> GSPAKIKIVAPLESALIPGGETYQLRCDIMSTPAATIHWKFNGKLIQGSNELNVEEKLLNFGKAIVDTGIVASILTIQCPSAENSGTYSCVGYNGHQTIETVAEVEIEGEASGCRSNHKSAPEIVFWTDSRFEMTGNVATLVCRANQQVDWVW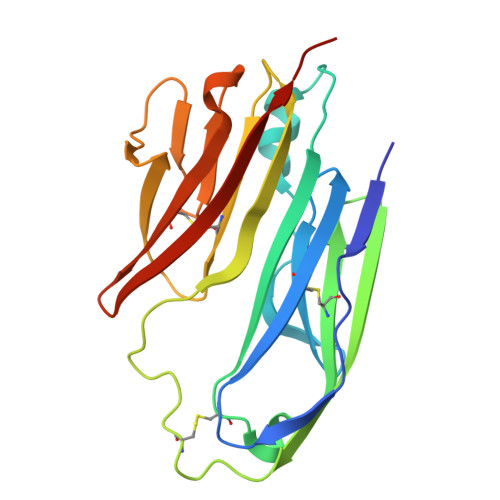MSNDELVKNNDKFTVLSNGDLVIKNIVWDDMGTYTCIARNQFGEARQETFLYPTAHHHHHH>HHHHHHFNLPPGNYKKPKLL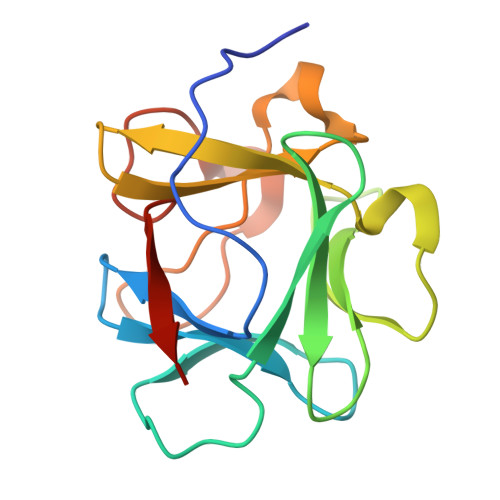YCSNGGHFLRILPDGTVDGTRDRSDQHIQLQLSAESVGEVYIKSTETGQYLAMDTDGLLYGSQTPNEECLFLERLEENHYNTYISKKHAEKNWFVGLKKNGSCKRGPRTHYGQKAILFLPLPVSSD[2x]> MADVINVSVNLEAFSQAISAIQALRSSVSRVFDCLKDGMRNKETLEGREKAFIAHFQDNLHSVNRDLNELERLSNLVGKPSENHPLHNSGLLSLDPVQDKTPLYSQLLQAYKWSNKLQYHAGLASGLLNQQSLKRSANQMGVSAKRRPKAQPTTLVLPPQYVDDVISRIDRMFPEMSIHLSRPNGTSAMLLVTLGKVLKVIVVMRSLFIDRTIVKGYNENVYTEDGKLDIWSKSNYQVFQKVTDHATTALLHYQLPQMPDVVVRSFMTWLRSYIKLFQAPCQRCGKFLQDGLPPTWRDFRTLEAFHDTCRQ;> MAAPLGGMFSGQPPGPPQAPPGLPGQASLLQAAPGAPRPSSSTLVDELESSFEACFASLVSQDYVNGTDQEEIRTGVDQCIQKFLDIARQTECFFLQKRLQLSVQKPEQVIKEDVSELRNELQRKDALVQKHLTKLRHWQQVLEDINVQHKKPADIPQGSLAYLEQASANIPAPLKPT;> MAASQQQASAASSAAGVSGPSSAGGPGPQQQPQPPAQLVGPAQSGLLQQQQQDFDPVQRYKMLIPQLKESLQTLMKVAAQNLIQNTNIDNGQKSSDGPIQRFDKCLEEFYALCDQLELCLRLAHECLSQSCDSAKHSPTLVPTATKPDAVQPDSLPYPQYLAVIKAQISCAKDIHTALLDCANKVTGKTPAPPAGPGGTL;> MSTPPLAASGMAPGPFAGPQAQQAAREVNTASLCRIGQETVQDIVYRTMEIFQLLRNMQLPNGVTYHTGTYQDRLTKLQDNLRQLSVLFRKLRLVYDKCNENCGGMDPIPVEQLIPYVEEDGSKNDDRAGPPRFASEERREIAEVNKKLKQKNQQLKQIMDQLRNLIWDINAMLAMRN;> MAAAVAMETDDAGNRLRFQLELEFVQCLANPNYLNFLAQRGYFKDKAFVNYLKYLLYWKDPEYAKYLKYPQCLHMLELLQYEHFRKELVNAQCAKFIDEQQILHWQHYSRKRMRLQQALAEQQQQNNTSGK;> MKAQGETEESEKLSKMSSLLERLHAKFNQNRPWSETIKLVRQVMEKRVVMSSGGHQHLVSCLETLQKALKVTSLPAMTDRLESIARQNGLGSHLSASGTECYITSDMFYVEVQLDPAGQLCDVKVAHHGENPVSCPELVQQLREKNFDEFSKHLKGLVNLYNLPGDNKLKTKMYLALQSLEQDLSKMAIMYWKATNAGPLDKILHGSVGYLTPRSGGHLMNLKYYVSPSDLLDDKTASPIILHENNVSRSLGMNASVTIEGTSAVYKLPIAPLIMGSHPVDNKWTPSFSSITSANSVDLPACFFLKFPQPIPVSRAFVQKLQNCTGIPLFETQPTYAPLYELITQFELSKDPDPIPLNHNMRFYAALPGQQHCYFLNKDAPLPDGRSLQGTLVSKITFQHPGRVPLILNLIRHQVAYNTLIGSCVKRTILKEDSPGLLQFEVCPLSESRFSVSFQHPVNDSLVCVVMDVQDSTHVSCKLYKGLSDALICTDDFIAKVVQRCMSIPVTMRAIRRKAETIQADTPALSLIAETVEDMVKKNLPPASSPGYGMTTGNNPMSGTTTPTNTFPGGPITTLFNMSMSIKDRHESVGHGEDFSKVSQNPILTSLLQITGNGGSTIGSSPTPPHHTPPPVSSMAGNTKNHPMLMNLLKDNPAQDFSTLYGSSPLERQNSSSGSPRMEICSGSNKTKKKKSSRLPPEKPKHQTEDDFQRELFSMDVDSQNPIFDVNMTADTLDTPHITPAPSQCSTPPTTYPQPVPHPQPSIQRMVRLSSSDSIGPDVTDILSDIAEEASKLPSTSDDCPAIGTPLRDSSSSGHSQSTLFDSDVFQTNNNENPYTDPADLIADAAGSPSSDSPTNHFFHDGVDFNPDLLNSQSQSGFGEEYFDESSQSGDNDDFKGFASQALNTLGVPMLGGDNGETKFKGNNQADTVDFSIISVAGKALAPADLMEHHSGSQGPLLTTGDLGKEKTQKRVKEGNGTSNSTLSGPGLDSKPGKRSRTPSNDGKSKDKPPKRKKADTEGKSPSHSSSNRPFTPPTSTGGSKSPGSAGRSQTPPGVATPPIPKITIQIPKGTVMVGKPSSHSQYTSSGSVSSSGSKSHHSHSSSSSSSASTSGKMKSSKSEGSSSSKLSSSMYSSQGSSGSSQSKNSSQSGGKPGSSPITKHGLSSGSSSTKMKPQGKPSSLMNPSLSKPNISPSHSRPPGGSDKLASPMKPVPGTPPSSKAKSPISSGSGGSHMSGTSSSSGMKSSSGLGSSGSLSQKTPPSSNSCTASSSSFSSSGSSMSSSQNQHGSSKGKSPSRNKKPSLTAVIDKLKHGVVTSGPGGEDPLDGQMGVSTNSSSHPMSSKHNMSGGEFQGKREKSDKDKSKVSTSGSSVDSSKKTSESKNVGSTGVAKIIISKHDGGSPSIKAKVTLQKPGESSGEGLRPQMASSKNYGSPLISGSTPKHERGSPSHSKSPAYTPQNLDSESESGSSIAEKSYQNSPSSDDGIRPLPEYSTEKHKKHKKEKKKVKDKDRDRDRDKDRDKKKSHSIKPESWSKSPISSDQSLSMTSNTILSADRPSRLSPDFMIGEEDDDLMDVALIGN;> MAASSSGEKEKERLGGGLGVAGGNSTRERLLSALEDLEVLSRELIEMLAISRNQKLLQAGEENQVLELLIHRDGEFQELMKLALNQGKIHHEMQVLEKEVEKRDSDIQQLQKQLKEAEQILATAVYQAKEKLKSIEKARKGAISSEEIIKYAHRISASNAVCAPLTWVPGDPRRPYPTDLEMRSGLLGQMNNPSTNGVNGHLPGDALAAGRLPDVLAPQYPWQSNDMSMNMLPPNHSSDFLLEPPGHNKENEDDVEIMSTDSSSSSSESD;> MAAVDIRDNLLGISWVDSSWIPILNSGSVLDYFSERSNPFYDRTCNNEVVKMQRLTLEHLNQMVGIEYILLHAQEPILFIIRKQQRQSPAQVIPLADYYIIAGVIYQAPDLGSVINSRVLTAVHGIQSAFDEAMSYCRYHPSKGYWWHFKDHEEQDKVRPKAKRKEEPSSIFQRQRVDALLLDLRQKFPPKFVQLKPGEKPVPVDQTKKEAEPIPETVKPEEKETTKNVQQTVSAKGPPEKRMRLQ;> MGEPQQVSALPPPPMQYIKEYTDENIQEGLAPKPPPPIKDSYMMFGNQFQCDDLIIRPLESQGIERLHPMQFDHKKELRKLNMSILINFLDLLDILIRSPGSIKREEKLEDLKLLFVHVHHLINEYRPHQARETLRVMMEVQKRQRLETAERFQKHLERVIEMIQNCLASLPDDLPHSEAGMRVKTEPMDADDSNNCTGQNEHQRENSGHRRDQIIEKDAALCVLIDEMNERP;> MQREEKQLEASLDALLSQVADLKNSLGSFICKLENEYGRLTWPSVLDSFALLSGQLNTLNKVLKHEKTPLFRNQVIIPLVLSPDRDEDLMRQTEGRVPVFSHEVVPDHLRTKPDPEVEEQEKQLTTDAARIGADAAQKQIQSLNKMCSNLLEKISKEERESESGGLRPNKQTFNPTDTNALVAAVAFGKGLSNWRPSGSSGPGQAGQPGAGTILAGTSGLQQVQMAGAPSQQQPMLSGVQMAQAGQPGKMPSGIKTNIKSASMHPYQR;> MASAGVAAGRQAEDVLPPTSDQPLPDTKPLPPPQPPPVPAPQPQQSPAPRPQSPARAREEENYSFLPLVHNIIKCMDKDSPEVHQDLNALKSKFQEMRKLISTMPGIHLSPEQQQQQLQSLREQVRTKNELLQKYKSLCMFEIPKE;> MAEKFDHLEEHLEKFVENIRQLGIIVSDFQPSSQAGLNQKLNFIVTGLQDIDKCRQQLHDITVPLEVFEYIDQGRNPQLYTKECLERALAKNEQVKGKIDTMKKFKSLLIQELSKVFPEDMAKYRSIRGEDHPPS;> MATYSLANERLRALEDIEREIGAILQNAGTVILELSKEKTNERLLDRQAAAFTASVQHVEAELSAQIRYLTQVATGQPHEGSSYSSRKDCQMALKRVDYARLKLSDVARTCEQMLEN;> MAPVQLENHQLVPPGGGGGGSGGPPSAPAPPPPGAAVAAAAAAAASPGYRLSTLIEFLLHRAYSELMVLTDLLPRKSDVERKIEIVQFASRTRQLFVRLLALVKWANNAGKVEKCAMISSFLDQQAILFVDTADRLASLARDALVHARLPSFAIPYAIDVLTTGSYPRLPTCIRDKIIPPDPITKIEKQATLHQLNQILRHRLVTTDLPPQLANLTVANGRVKFRVEGEFEATLTVMGDDPDVPWRLLKLEILVEDKETGDGRALVHSMQISFIHQLVQSRLFADEKPLQDMYNCLHSFCLSLQLEVLHSQTLMLIRERWGDLVQVERYHAGKCLSLSVWNQQVLGRKTGTASVHKVTIKIDENDVSKPLQIFHDPPLPASDSKLVERAMKIDHLSIEKLLIDSVHARAHQKLQELKAILRGFNANENSSIETALPALVVPILEPCGNSECLHIFVDLHSGMFQLMLYGLDQATLDDMEKSVNDDMKRIIPWIQQLKFWLGQQRCKQSIKHLPTISSETLQLSNYSTHPIGNLSKNKLFIKLTRLPQYYIVVEMLEVPNKPTQLSYKYYFMSVNAADREDSPAMALLLQQFKENIQDLVFRTKTGKQTRTNAKRKLSDDPCPVESKKTKRAGEMCAFNKVLAHFVAMCDTNMPFVGLRLELSNLEIPHQGVQVEGDGFSHAIRLLKIPPCKGITEETQKALDRSLLDCTFRLQGRNNRTWVAELVFANCPLNGTSTREQGPSRHVYLTYENLLSEPVGGRKVVEMFLNDWNSIARLYECVLEFARSLPDIPAHLNIFSEVRVYNYRKLILCYGTTKGSSISIQWNSIHQKFHISLGTVGPNSGCSNCHNTILHQLQEMFNKTPNVVQLLQVLFDTQAPLNAINKLPTVPMLGLTQRTNTAYQCFSILPQSSTHIRLAFRNMYCIDIYCRSRGVVAIRDGAYSLFDNSKLVEGFYPAPGLKTFLNMFVDSNQDARRRSVNEDDNPPSPIGGDMMDSLISQLQPPPQQQPFPKQPGTSGAYPLTSPPTSYHSTVNQSPSMMHTQSPGNLHAASSPSGALRAPSPASFVPTPPPSSHGISIGPGASFASPHGTLDPSSPYTMVSPSGRAGNWPGSPQVSGPSPAARMPGMSPANPSLHSPVPDASHSPRAGTSSQTMPTNMPPPRKLPQRSWAASIPTILTHSALNILLLPSPTPGLVPGLAGSYLCSPLERFLGSVIMRRHLQRIIQQETLQLINSNEPGVIMFKTDALKCRVALSPKTNQTLQLKVTPENAGQWKPDELQVLEKFFETRVAGPPFKANTLIAFTKLLGAPTHILRDCVHIMKLELFPDQATQLKWNVQFCLTIPPSAPPIAPPGTPAVVLKSKMLFFLQLTQKTSVPPQEPVSIIVPIIYDMASGTTQQADIPRQQNSSVAAPMMVSNILKRFAEMNPPRQGECTIFAAVRDLMANLTLPPGGRP;> MDVSGQETDWRSTAFRQKLVSQIEDAMRKAGVAHSKSSKDMESHVFLKAKTRDEYLSLVARLIIHFRDIHNKKSQASVSDPMNALQSLTGGPAAGAAGIGMPPRGPGQSLGGMGSLGAMGQPMSLSGQPPPGTSGMAPHSMAVVSTATPQTQLQLQQVALQQQQQQQQFQQQQQAALQQQQQQQQQQQFQAQQSAMQQQFQAVVQQQQQLQQQQQQQQHLIKLHHQNQQQIQQQQQQLQRIAQLQLQQQQQQQQQQQQQQQQALQAQPPIQQPPMQQPQPPPSQALPQQLQQMHHTQHHQPPPQPQQPPVAQNQPSQLPPQSQTQPLVSQAQALPGQMLYTQPPLKFVRAPMVVQQPPVQPQVQQQQTAVQTAQAAQMVAPGVQMITEALAQGGMHIRARFPPTTAVSAIPSSSIPLGRQPMAQVSQSSLPMLSSPSPGQQVQTPQSMPPPPQPSPQPGQPSSQPNSNVSSGPAPSPSSFLPSPSPQPSQSPVTARTPQNFSVPSPGPLNTPVNPSSVMSPAGSSQAEEQQYLDKLKQLSKYIEPLRRMINKIDKNEDRKKDLSKMKSLLDILTDPSKRCPLKTLQKCEIALEKLKNDMAVPTPPPPPVPPTKQQYLCQPLLDAVLANIRSPVFNHSLYRTFVPAMTAIHGPPITAPVVCTRKRRLEDDERQSIPSVLQGEVARLDPKFLVNLDPSHCSNNGTVHLICKLDDKDLPSVPPLELSVPADYPAQSPLWIDRQWQYDANPFLQSVHRCMTSRLLQLPDKHSVTALLNTWAQSVHQACLSAA;> MCDLRRPAAGGMMDLAYVCEWEKWSKSTHCPSVPLACAWSCRNLIAFTMDLRSDDQDLTRMIHILDTEHPWDLHSIPSEHHEAITCLEWDQSGSRLLSADADGQIKCWSMADHLANSWESSVGSLVEGDPIVALSWLHNGVKLALHVEKSGASSFGEKFSRVKFSPSLTLFGGKPMEGWIAVTVSGLVTVSLLKPSGQVLTSTESLCRLRGRVALADIAFTGGGNIVVATADGSSASPVQFYKVCVSVVSEKCRIDTEILPSLFMRCTTDLNRKDKFPAITHLKFLARDMSEQVLLCASSQTSSIVECWSLRKEGLPVNNIFQQISPVVGDKQPTILKWRILSATNDLDRVSAVALPKLPISLTNTDLKVASDTQFYPGLGLALAFHDGSVHIVHRLSLQTMAVFYSSAAPRPVDEPAMKRPRTAGPAVHLKAMQLSWTSLALVGIDSHGKLSVLRLSPSMGHPLEVGLALRHLLFLLEYCMVTGYDWWDILLHVQPSMVQSLVEKLHEEYTRQTAALQQVLSTRILAMKASLCKLSPCTVTRVCDYHTKLFLIAISSTLKSLLRPHFLNTPDKSPGDRLTEICTKITDVDIDKVMINLKTEEFVLDMNTLQALQQLLQWVGDFVLYLLASLPNQGSLLRPGHSFLRDGTSLGMLRELMVVIRIWGLLKPSCLPVYTATSDTQDSMSLLFRLLTKLWICCRDEGPASEPDEALVDECCLLPSQLLIPSLDWLPASDGLVSRLQPKQPLRLQFGRAPTLPGSAATLQLDGLARAPGQPKIDHLRRLHLGACPTEECKACTRCGCVTMLKSPNRTTAVKQWEQRWIKNCLAVEGRGPDACVTSRASEEAPAFVQLGPQSTHHSPRTPRSLDHLHPEDRP;> MSGVRAVRISIESACEKQVHEVGLDGTETYLPPLSMSQNLARLAQRIDFSQGSGSEEEEAAGTEGDAQEWPGAGSSADQDDEEGVVKFQPSLWPWDSVRNNLRSALTEMCVLYDVLSIVRDKKFMTLDPVSQDALPPKQNPQTLQLISKKKSLAGAAQILLKGAERLTKSVTENQENKLQRDFNSELLRLRQHWKLRKVGDKILGDLSYRSAGSLFPHHGTFEVIKNTDLDLDKKIPEDYCPLDVQIPSDLEGSAYIKVSIQKQAPDIGDLGTVNLFKRPLPKSKPGSPHWQTKLEAAQNVLLCKEIFAQLSREAVQIKSQVPHIVVKNQIISQPFPSLQLSISLCHSSNDKKSQKFATEKQCPEDHLYVLEHNLHLLIREFHKQTLSSIMMPHPASAPFGHKRMRLSGPQAFDKNEINSLQSSEGLLEKIIKQAKHIFLRSRAAATIDSLASRIEDPQIQAHWSNINDVYESSVKVLITSQGYEQICKSIQLQLNIGVEQIRVVHRDGRVITLSYQEQELQDFLLSQMSQHQVHAVQQLAKVMGWQVLSFSNHVGLGPIESIGNASAITVASPSGDYAISVRNGPESGSKIMVQFPRNQCKDLPKSDVLQDNKWSHLRGPFKEVQWNKMEGRNFVYKMELLMSALSPCLL;> MEAPPVTMMPVTGGTINMMEYLLQGSVLDHSLESLIHRLRGLCDNMEPETFLDHEMVFLLKGQQASPFVLRARRSMDRAGAPWHLRYLGQPEMGDKNRHALVRNCVDIATSENLTDFLMEMGFRMDHEFVAKGHLFRKGIMKIMVYKIFRILVPGNTDSTEALSLSYLVELSVVAPAGQDMVSDDMKNFAEQLKPLVHLEKIDPKRLM;> MENFTALFGAQADPPPPPTALGFGPGKPPPPPPPPAGGGPGTAPPPTAATAPPGADKSGAGCGPFYLMRELPGSTELTGSTNLITHYNLEQAYNKFCGKKVKEKLSNFLPDLPGMIDLPGSHDNSSLRSLIEKPPILSSSFNPITGTMLAGFRLHTGPLPEQCRLMHIQPPKKKNKHKHKQSRTQDPVPPETPSDSDHKKKKKKKEEDPDRKRKKKEKKKKKNRHSPDHPGMGSSQASSSSSLR;> MGVTCVSQMPVAEGKSVQQTVELLTRKLEMLGAEKQGTFCVDCETYHTAASTLGSQGQTGKLMYVMHNSEYPLSCFALFENGPCLIADTNFDVLMVKLKGFFQSAKASKIETRGTRYQYCDFLVKVGTVTMGPSARGISVEVEYGPCVVASDCWSLLLEFLQSFLGSHTPGAPAVFGNRHDAVYGPADTMVQYMELFNKIRKQQQVPVAGIR;> MADRLTQLQDAVNSLADQFCNAIGVLQQCGPPASFNNIQTAINKDQPANPTEEYAQLFAALIARTAKDIDVLIDSLPSEESTAALQAASLYKLEEENHEAATCLEDVVYRGDMLLEKIQSALADIAQSQLKTRSGTHSQSLPDS;> MAQQRALPQSKETLLQSYNKRLKDDIKSIMDNFTEIIKTAKIEDETQVSRATQGEQDNYEMHVRAANIVRAGESLMKLVSDLKQFLILNDFPSVNEAIDQRNQQLRTLQEECDRKLITLRDEISIDLYELEEEYYSSSSSLCEANDLPLCEAYGRLDLDTDSADGLSAPLLASPEPSAGPLQVAAPAHSHAGGPGPTEHA;> METQLQSIFEEVVKTEVIEEAFPGMFMDTPEDEKTKLISCLGAFRQFWGGLSQESHEQCIQWIVKFIHGQHSPKRISFLYDCLAMAVETGLLPPRLVCESLINSDTLEWERTQLWALTFKLVRKIIGGVDYKGVRDLLKVILEKILTIPNTVSSAVVQQLLAAREVIAYILERN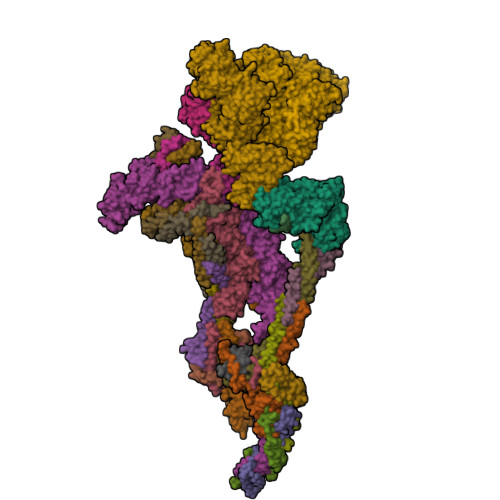ACLLPAYFAVTEIRKLYPEGKLPHWLLGNLVSDFVDTFRPTARINSICGRCSLLPVVNNSGAICNSWKLDPATLRFPLKGLLPYDKDLFEPQTALLRYVLEQPYSRDMVCNMLGLNKQHKQRCPVLEDQLVDLVVYAMERSETEEKFDDGGTSQLLWQHLSSQLIFFVLFQFASFPHMVLSLHQKLAGRGLIKGRDHLMWVLLQFISGSIQKNALADFLPVMKLFDLLYPEKEYIPVPDINKPQSTHAFAMTCIWIHLNRKAQNDNSKLQIPIPHSLRLHHEFLQQSLRNKSLQMNDYKIALLCNAYSTNSECFTLPMGALVETIYGNGIMRIPLPGTNCMASGSITPLPMNLLDSLTVHAKMSLIHSIATRVIKLAHAKSSVALAPALVETYSRLLVYMEIESLGIKGFISQLLPTVFKSHAWGILHTLLEMFSYRMHHIQPHYRVQLLSHLHTLAAVAQTNQNQLHLCVESTALRLITALGSSEVQPQFTRFLSDPKTVLSAESEELNRALILTLARATHVTDFFTGSDSIQGTWCKDILQTIMSFTPHNWASHTLSCFPGPLQAFFKQNNVPQESRFNLKKNVEEEYRKWKSMSNENDIITHFSMQGSPPLFLCLLWKMLLETDHINQIGYRVLERIGARALVAHVRTFADFLVYEFSTSAGGQQLNKCIEILNDMVWKYNIVTLDRLILCLAMRSHEGNEAQVCYFIIQLLLLKPNDFRNRVSDFVKENSPEHWLQNDWHTKHMNYHKKYPEKLYFEGLAEQVDPPVQIQSPYLPIYFGNVCLRFLPVFDIVIHRFLELLPVSKSLETLLDHLGGLYKFHDRPVTYLYNTLHYYEMHLRDRAFLKRKLVHAIIGSLKDNRPQGWCLSDTYLKCAMNAREENPWVPDDTYYCRLIGRLVDTMAGKSPGPFPNCDWRFNEFPNPAAHALHVTCVELMALAVSGKEVGNALLNVVLKSQPLVPRENITAWMNAIGLIITALPEPYWIVLHDRIVSVISSPSLTSETEWVGYPFRLFDFTACHQSYSEMSCSYTLALAHAVWHHSSIGQLSLIPKFLTEVLLPIVKTEFQLLYVYHLVGPFLQRFQQERTRCMIEIGVAFYDMLLNVDQCSTHLNYMDPICDFLYHMKYMFTGDSVKEQVEKIICNLKPALKLRLRFITHISKMEPAAVPPQAMNSGSPAPQSNQVPVSLPVTQ;> MKVVNLKQAILQAWKERWSDYQWAINMKKFFPKGATWDILNLADALLEQAMIGPSPNPLILSYLKYAISSQMVSYSSVLTAISKFDDFSRDLCVQALLDIMDMFCDRLSCHGKAEECIGLCRALLSALHWLLRCTAASAERLREGLEAGTPAAGEKQLAMCLQRLEKTLSSTKNRALLHIAKLEEASSWTAIEHSLLKLGEILANLSNPQLRSQAEQCGTLIRSIPTMLSVHAEQMHKTGFPTVHAVILLEGTMNLTGETQSLVEQLTMVKRMQHIPTPLFVLEIWKACFVGLIESPEGTEELKWTAFTFLKIPQVLVKLKKYSHGDKDFTEDVNCAFEFLLKLTPLLDKADQRCNCDCTNFLLQECGKQGLLSEASVNNLMAKRKADREHAPQQKSGENANIQPNIQLILRAEPTVTNILKTMDADHSKSPEGLLGVLGHMLSGKSLDLLLAAAAATGKLKSFARKFINLNEFTTYGSEESTKPASVRALLFDISFLMLCHVAQTYGSEVILSESRTGAEVPFFETWMQTCMPEEGKILNPDHPCFRPDSTKVESLVALLNNSSEMKLVQMKWHEACLSISAAILEILNAWENGVLAFESIQKITDNIKGKVCSLAVCAVAWLVAHVRMLGLDEREKSLQMIRQLAGPLFSENTLQFYNERVVIMNSILERMCADVLQQTATQIKFPSTGVDTMPYWNLLPPKRPIKEVLTDIFAKVLEKGWVDSRSIHIFDTLLHMGGVYWFCNNLIKELLKETRKEHTLRAVELLYSIFCLDMQQVTLVLLGHILPGLLTDSSKWHSLMDPPGTALAKLAVWCALSSYSSHKGQASTRQKKRHREDIEDYISLFPLDDVQPSKLMRLLSSNEDDANILSSPTDRSMSSSLSASQLHTVNMRDPLNRVLANLFLLISSILGSRTAGPHTQFVQWFMEECVDCLEQGGRGSVLQFMPFTTVSELVKVSAMSSPKVVLAITDLSLPLGRQVAAKAIAAL;> MTAAPASPQQIRDRLLQAIDPQSNIRNMVAVLEVISSLEKYPITKEALEETRLGKLINDVRKKTKNEELAKRAKKLLRSWQKLIEPAHQHEAALRGLAGATGSANGGAHNCRPEVGAAGPPRSIHDLKSRNDLQRLPGQRLDRLGSRKRRGDQRDLGHPGPPPKVSKASHDPLVPNSSPLPTNGISGSPESFASSLDGSGHAGPEGSRLERDENDKHSGKIPVNAVRPHTSSPGLGKPPGPCLQPKASVLQQLDRVDETPGPPHPKGPPRCSFSPRNSRHEGSFARQQSLYAPKGSVPSPSPRPQALDATQVPSPLPLAQPSTPPVRRLELLPSAESPVCWLEQPESHQRLAGPGCKAGLSPAEPLLSRAGFSPDSSKADSDAASSGGSDSKKKKRYRPRDYTVNLDGQVAEAGVKPVRLKERKLTFDPMTRQIKPLTQKEPVRADSPVHMEQQSRTELDKQEAKASLQSPFEQTNWKELSRNEIIQSYLSRQSSLLSSSGAQTPGAHHFMSEYLKQEESTRQGARQLHVLVPQSPPTDLPGLTREVTQDDLDRIQASQWPGVNGCQDTQGNWYDWTQCISLDPHGDDGRLNILPYVCLD>[3x]PPGPPGPPGA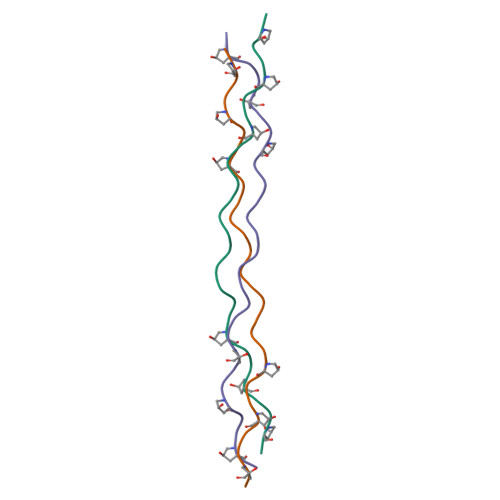NGLSGERGPPGPPGPPG>[2x]MAHHHHHHMTTLKNDRFLRAL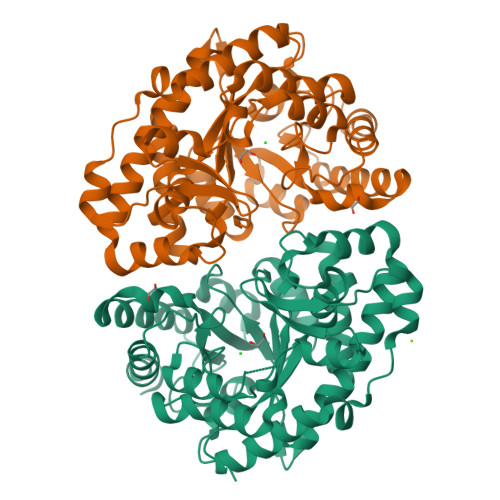LREPVDTTPIWMMRQAGRYLPEYRETRSKAGDFLSLCKNTEFACEVTLQPLRRYDLDAAILFSDILTIPDALGLGLYFETGEGPKFHKTVRTEQDVANLPKLNAKADLDYVMNAVSTIRSALGGQVPLIGFSGSPWTLATYMVEGGSSKEFRFTKQMMYAQPEVLHALLDHLADSVIDYLNAQIDAGAQAIQIFDSWGGALAHREYVEFSLNYMKKIIAGLQREKDGRRIPVIVFTKGGGQWLEPMITTGADALGLDWTTPLNTARTTVAGRVALQGNLDPAVLYGSAASIEKAVKAMLDDAYANGEKTGYVANLGHGITQWVDPAQPKIFVDTVHEYSAKYLG2-{[3-(3,4-dimethylphenoxy)phenyl]carbamoyl}-4-nitrobenzoic acid | 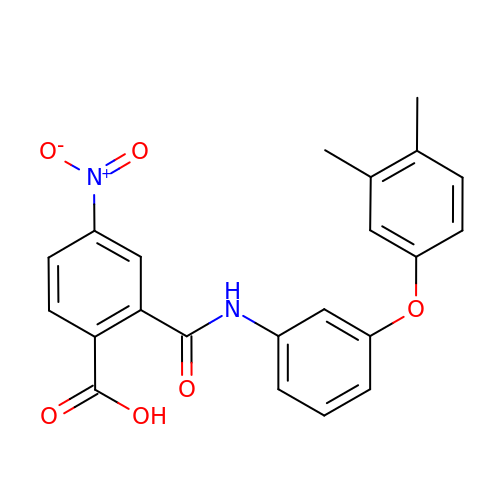C22 H18 N2 O6 | GQGBAJUULMBPOF-UHFFFAOYSA-N> DGKKKKK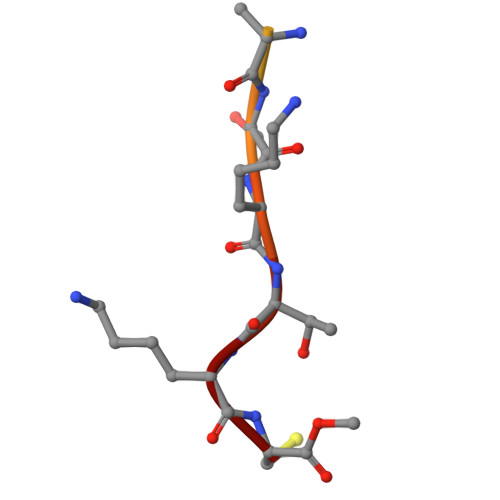KSKTKC> MILMIDNYDSFTYNLVQYLGELGEEVVVYRNDEITIAEIEKLKPDHLVISPGPCTPNEAGISLEVIKHFAGKIPILGVCL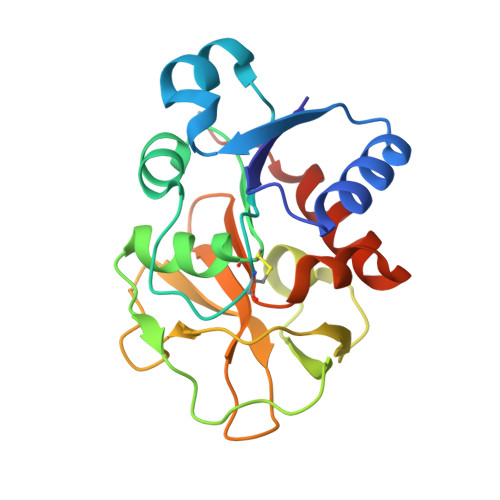GHQSIGQAFGGKIVRAKQVMHGKTSEIYHNNKGVFKGLNNPFEATRYHSLVVERETLPDCLEITAWTETDEGEIMGIRHKTLPIEGVQFHPESILTEQGHELLKNFLKELEHHHHHH>[4x]MHHHHHHITSLYKKAGMPIWSSHAPYGSFSRDGYSWNNDVWGPRPGPQTISVSGVNRWSVW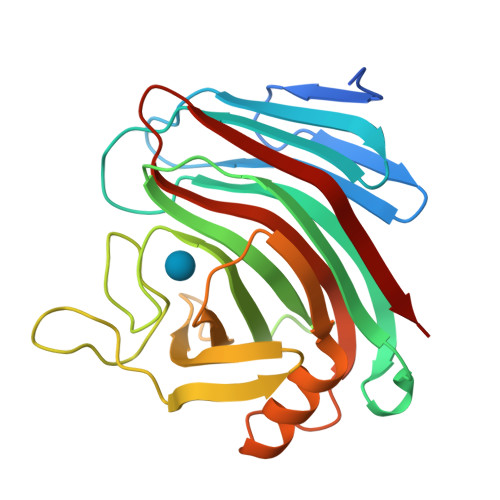SDQPNTPGIKSYPHVAFNIGKPLSSINTLSSSFNQEVPTGGAWDVAYDIWDSSNKHEIMLWTNYTGNSDGSGNVKPISYHYAPSGAAIPVYSNVNVGGATWNVFEGEGPDGHKVISLLRTSKTNSGTVDIKSILQWIKSKGYFGDIEVGSVQYGVEITSSPGGKNFNFNNWSVTSK[(2R)-2-hydroxypropyl]phosphonic acid | C3 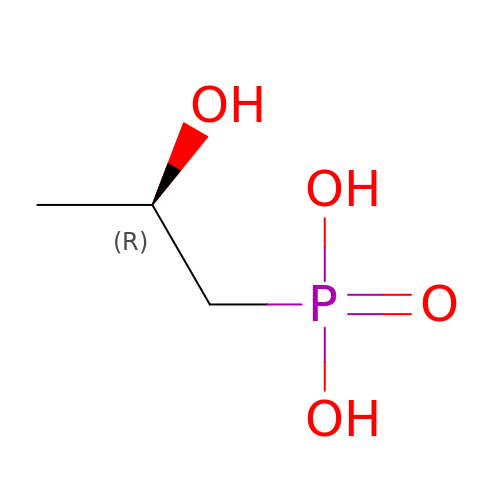H9 O4 P | ZFVCONUOLQASEW-GSVOUGTGSA-N1-(5-ethoxypyridin-3-yl)-1,4-diazepane | C12 H19 N3 O | 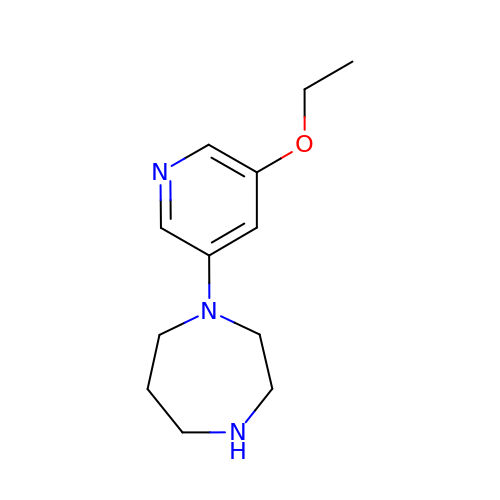RQXFSCANOMMTFZ-UHFFFAOYSA-N>[2x]MGH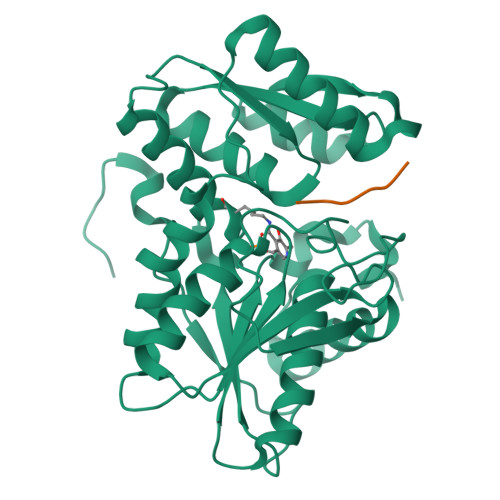HHHHHMAQKPVDNITQIIGGTPVVKLRNVVDDNAADVYVKLEYQNPGGSVKDRIALAMIEKAEREGKIKPGDTIVEPTSGNTGIGLAFVCAAKGYKAVFTMPETMSQERRNLLKAYGAELVLTPGSEAMKGAIKKAKELKEEHGYFEPQQFENPANPEVHELTTGPELLQQFEGKTIDAFLAGVGTGGTLSGVGKVLKKEYPNIEIVAIEPEASPVLSGGEPGPHKLQGLGAGFIPGTLNTEIYDSIIKVGNDTAMEMSRRVAKEEGILAGISSGAAIYAAIQKAKELGKGKTVVTVLPSNGERYLSTPLYSFDD;>[2x]EDLDGYMFYI5-[(5S,9R)-9-(4-CYANOPHENYL)-3-(3,5-DICHLOROPHENYL)-1-METHYL-2,4-DIOXO-1,3,7-TRIAZASPIRO [4.4]NON-7-YL]METHYL]-3-THIOPHENECARBOXYLICACID | C26 H20 Cl2 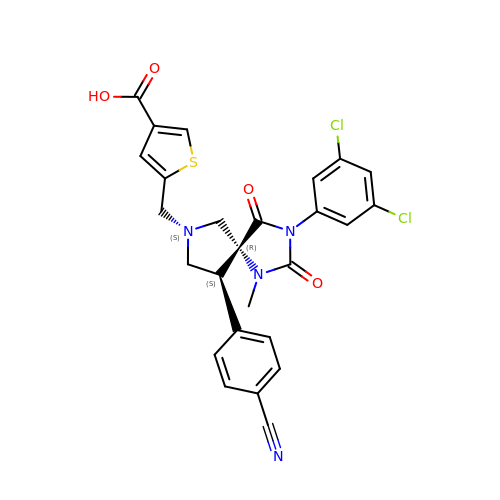N4 O4 S | NXNKJLOEGWSJGI-BKMJKUGQSA-N> GPAMPPILDVIVIGGGQAALTTAYFLRRTSLSYLLLDEQPGPGGAWLHAWDSLRLFSPAAWSSIAGWPMPSPTEPGNPTRNDVIDYLRRYEDRYQFPIQRPVRVDTVTRLDDLWRVQAGDQQWLARAVISATGTWSKPFIPPYEGRELFQGAQIHSAHYRTPAPFAGKRVMVVGGGNSGAQVLAELSSVSETLWITQEPPAFLPDEVDGRVLFERATARWKAQQEGRSIDEPAGGFGDIVMVPPVREARERGVLVAERPFARFTETGVEWADGRRENLDAVIWCSGFRPALDHLRELGVVEADGKVQVEDTRVVKQPNLWLVGYGDWTGMASATLIGVTRTARSTADQVVQALTATPSRRP

FMOs typically employ the phosphorylated nicotinamide cofactor NADPH to reduce a molecule of FAD within the enzyme, which then reacts with molecular oxygen to form a (hydro)peroxy flavin species that is the catalytic oxidant in reaction. Natural variation within the phosphate binding region, and its influence on nicotinamide cofactor promiscuity, was explored through the cloning, expression, characterisation and structural studies of FMOs from Cellvibrio sp. BR (CFMO) and Pseudomonas stutzeri NF13 (PSFMO), which possess Thr–Ser and Gln–Glu in the putative phosphate recognition positions, respectively. The structures of CFMO and PSFMO revealed the context of the phosphate binding loop in each case, and also clarified the structure of the mobile helix–loop–helix motif that appears to shield the FAD-binding pocket from bulk solvent in this class of FMOs, a feature that was absent from the structure of SMFMO. In order to shed light on the nature of the cofactor binding loops in CFMO and PSFMO, the structures of each in complex with the flavin FAD were determined to resolutions of 2.39 Å and 1.83 Å, respectively.

Crystals of PSFMO grew in the P3221 space group, with one molecule in the asymmetric unit, although both size-exclusion studies (not shown), and the relationship of the monomer to its closest crystallographic symmetry partner, are strongly suggestive of an active dimer for PSFMO as with SMFMO and CFMO. Analysis of a dimer pair by PISA revealed an interfacial area of 955 Å2, with six H-bonds and 8 salt bridges formed between the monomers. In the case of PSFMO, there was electron density for each amino acid in the monomer from residue Met1 to Pro354, which allowed for the first time the observation of the entire backbone of the flexible helix–loop–helix structure, represented by residues 207–234 in PSFMO, and incorporating helices α9 and α10, over FAD that had been missing from SMFMO structures and only partially present in CFMO, although side-chain density for residues 222–227 was poor. The monomer of PSFMO superposed with the structure of the SMFMO with an r.m.s.d. of 0.90 Å over 327 Cα atoms. FAD was again clearly visible in the omit map after building and refinement of the protein atoms, and was also modelled and refined successfully in the oxidised form, the density revealing no puckering of the tricyclic ring system that might be indicative of the reduced flavin. The nucleotide binding site of PSFMO featured a glycerol molecule, from the cryoprotectant, occupying approximately the same position as the adenine ring of NADPH in mFMO, and with the hydroxyl groups forming hydrogen bonds with the side chain of Tyr140, the backbone NH of Gln194 and a water molecule. Superimposition of the putative phosphate binding sites of SMFMO and PSFMO revealed that the backbone Cα atoms of residues thought to be responsible for cofactor promiscuity in SMFMO, Gln193 and His194, are in the same position as those in PSFMO, Gln194 and Glu195.In E. coli, the ssuABC and tauABC gene products encode for an ABC transporter for the uptake of alkanesulfonates and taurine, respectively; TauA is the SBP that recognizes and binds taurine, TauBC is the ABC transporter that mediates the transport of taurine in an ATP-dependent manner. The SsuA and TauA proteins belong to the class II SBPs that are characterized by two globular domains, linked by a flexible linker, that form a cleft where the substrate binds. TauA is composed of two α/β-domains (domain I (23–104 and 202–319) and domain II (105–201)) connected by two-loop hinge regions (103–106 and 200–202) with the substrate-binding site located at the interface of the two domains; both domains are composed of five β-strands flanked by 11 and 4 α-helices, respectively. Although, SBPs are usually described as highly specific for their substrate, we show that TauA is capable of binding different taurine analogues and alkanesulfonates, including phosphonate analogues, with different affinities.

2-Aminoethylphosphonic acid (2-AEP) was selected as a structural analogue since it contains a phosphonate group instead of sulfonate. Although, 2-AEP has the same structural configuration as taurine, very weak binding could be measured, Kd of 649 µM, between TauA and 2-AEP. Despite the very low binding affinity between TauA and 2-AEP by ITC, a complex could be formed under crystallisation conditions. The 2-AEP is co-ordinated in a similar manner as taurine with an additional hydrogen bond between the phosphonate group and the side chain of Ser109. This hydrogen bond is absent from the taurine complex and it is a result of the different rotamer that Ser109 adopts in the presence of 2-AEP in order to co-ordinate the smaller phosphonate anion. SBPs have to undergo large conformational changes between the apo and substrate-bound states driven by ligand binding and in the case of 2-AEP, it is likely that 2-AEP binding that is also coupled to local conformational changes at the binding site, Ser109, is unfavourable, thus allowing the TauA to distinguish over smaller ligands. The crystal structure of TauA with 2-AEP suggests that although the phosphonate group has the same tetrahedral coordination as sulfonate, it cannot be effectively co-ordinated in the binding site and that the ethylamine group alone is not sufficient to co-ordinate tight binding of 2-AEP to taurine. The internuclear distance for the sulfate and phosphate anions has been determined to be 0.38 nm for S-O and 0.36 nm for P-O suggesting that the smaller 2-AEP phosphonate ionic radius results in weaker interactions with the binding site of TauA. Despite the high structural similarity between taurine and 2-AEP, the later also displaces 10 water molecules.

>MVNVTVAYQTSAEPAKVAQADNTFAKESGATVDWRKFDSGASIVRALASGDVQIGNLGSSPLAVAASQQVPIEVFLLASKLGNSEALVVKKTISKPEDLIGKRIAVPFISTTHYSLLAALKHWGIKPGQVEIVNLQPPAIIAAWQRGDIDGAYVWAPAVNALEKDGKVLTDSEQVGQWGAPTLDVWVVRKDFAEKHPEVVKAFAKSAIDAQQPYIANPDVWLKQPENISKLARLSGVPEGDVPGLVKGNTYLTPQQQTAELTGPVNKAIIDTAQFLKEQGKVPAVANDYSQYVTSRFV[2x]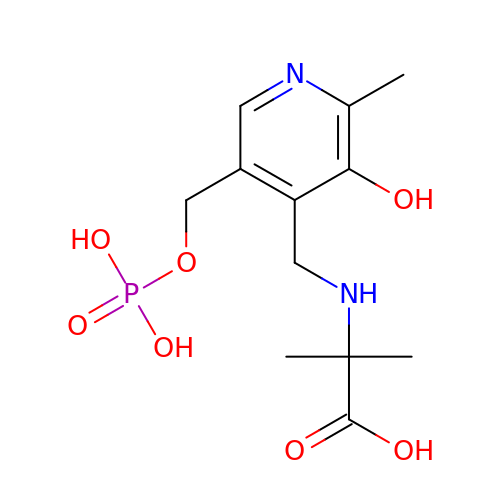N-[3-HYDROXY-2-METHYL-5-PHOSPHONOOXYMETHYL-PYRIDIN-4-YLMETHYL]-2-METHYLALANINE | C12 H19 N2 O7 P | NHGDGJKONAZETF-UHFFFAOYSA-N>[2x]MNHKVHHHHHHIEGRHMVSVEE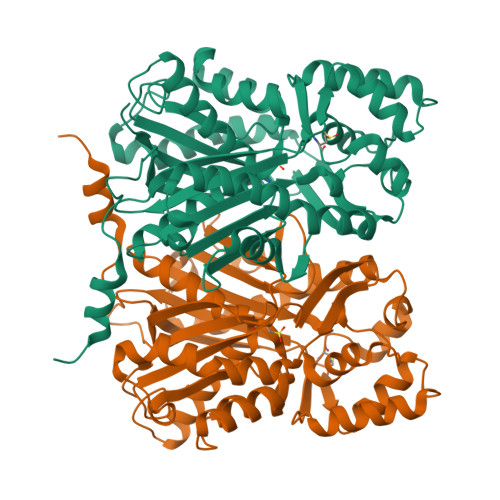IRKAQRAEGPATVMAIGTATPPNCVDQSTYPDYYFRITNSEHMTELKEKFKRMCDKSMIKKRYMYLNEEILKENPSVCAYMAPSLDARQDMVVVEVPKLGKEAATKAIKEWGQPKSKITHLIFCTTSGVDMPGADYQLTKLLGLRPSVKRYMMYQQGCFAGGTVLRLAKDLAENNKGARVLVVCSEITAVTFRGPTDTHLDSLVGQALFGDGAAAVIVGSDPLPVEKPLFQLVWTAQTILPDSEGAIDGHLREVGLTFHLLKDVPGLISKNIEKALVEAFQPLGISDYNSIFWIAHPGGPAILDQVEAKLGLKPEKMEATRHVLSEYGNMSSACVLFILDQMRKKSIENGLGTTGEGLDWGVLFGFGPGLTVETVVLRSVTL> MNQQKSLTLIVALTT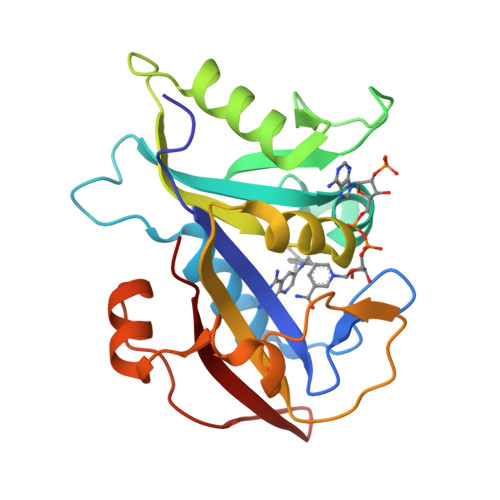SYGIGRSNSLPWKLKKEISYFKRVTSFVPTFDSFESMNVVLMGRKTWESIPLQNRPLKGRINVVITRNESLDLGNGIHSAKSLDHALELLYRTYGSESSVQINRIFVIGGAQLYKAAMDHPKLDRIMATIIYKDIHCDVFFPLKFRDKEWSSVWKKEKHSDLESWVGTKVPHGKINEDGFDYEFEMWTRDL>FACKTANGTAIPIGGGSANVYVNLAPVVNVGQNLVVDLSTQIFCHNDAPETITDYVTLQRGSAYGGVLSNFSGTVKYSGSSYPFPTTSETPRVVYNSRTDKPWPVALYLTPVSSAGGVAIKAGSLIA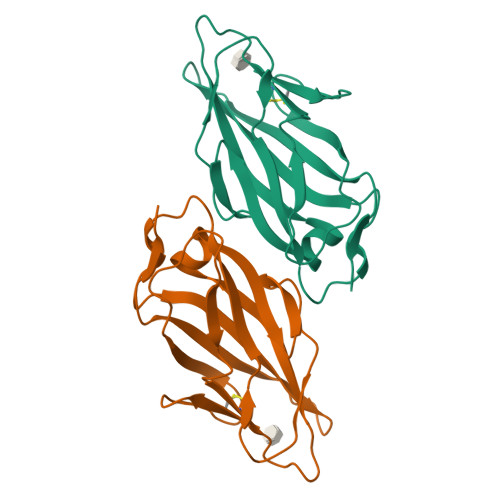VLILRQTNNYNSDDFQFVWNIYANNDVVVPT[2x]>TRDFN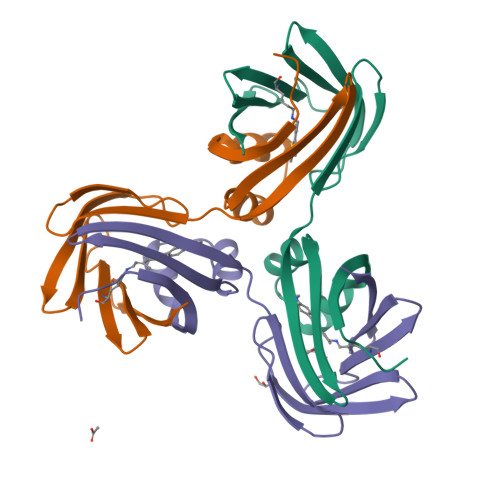GTWEMESNENFEGYMKALDIDFATRKIAVRLTFTDVIDQDGDNFKTKATSTFLNYDVDFTVGVEFDEYTKSLDNRHVKALVTWEGDVLVCVQKGEKENRGWKKWIEGDKLYLELTCGDQVCRQVFKKK[3x]Gloeobacter violaceus proton-gated ion channel (GLIC), a prokaryotic model of pLGICs, is particularly well-suited to stabilize preactive states under suboptimal activating conditions modulated by pH. The GLIC homomer consists of five subunits, each with an ECD and TMD. GLIC is activated by the protonation of a series of titratable residues in the ECD, leading to counterclockwise rotation and contraction of the ECD. Therefore, we established a data processing strategy involving symmetry expansion, backtracking particles, supervised particle reorientation, and 3D reconstruction to resolve high-resolution maps of various asymmetric intermediate states of nanodisc-reconstituted GLIC at pH 4.0, which provide comprehensive understanding of activation mechanism of GLIC.

Therefore, we generated F116A and Y251A mutants for cryo-EM study. The GLIC-F116A was reconstituted into nanodiscs at pH 2.5, a condition that stabilizes wild-type (WT) channels in an open conformation. The 3D classifications focused on a single subunit confirmed that all subunits exhibit i conformation. Therefore, the maps were reconstructed using both C1 and C5 symmetry with a nominal resolution of 2.53 and 2.14 Å, respectively. The structure shows an ECD conformation resembling the o5 state with RMSDCα of 0.28 Å, while the TMD closely aligns with the previously resolved resting state with RMSDCα of 0.39 Å. In the GLIC-F116A mutant, although the β1–β2 loop shows downward displacement, due to the absence of bulky side chain of F116 supported by a clear alanine density, the Pro-loop shows only subtle outward displacement, leaving the conformation of M2–M3 loop unaffected. This indicates that the bulky side chain of F116 is required for the outward displacement of the M2–M3 loop. Therefore, this structure highlights the critical role of F116 in transmitting ECD rearrangements to the TMD. Our results show that the ECD of the GLIC-F116A mutant adopts an open-like conformation, while the TMD remains in a resting-like state, indicating the channel is arrested in a preopen intermediate conformation.

>[5x]VSPPPPIADEPLTVNTGIYLIECYSLDDKAETFKVNAFLSLSWKDRRLAFDPVRSGVRVKTYEPEAIWIPEIRFVNVENARDADVVDISVSPDGTVQYLERFSARVLSPLDARRYPFDSQTLHIYLIVRSVDTRNIVLAVDLEKVGKNDDVFLTGWDIESFTAVVKPANFALEDRLESKLDYQLRISRQYFSYIPNIILPMLFILFISWTAFWSTSYEANVTLVVSTLIAHIAFNILVETNLPKTPYMTYTGAIIFMIYLFYFVAVIEVTVQHYLKVESQPARAASITRASRIAFPVVFLLANIILAFLFFG>[2x]MLIIGERINGMFGDIKRAIQERDPAPVQEWARRQEEGGARALDLNVGPAVQDKVSAMEWLVEVTQEVSNLTLCLDSTNIKAIEAGLKKCKNRA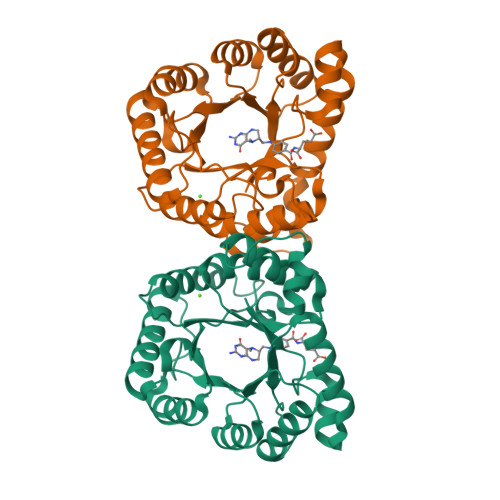MINSTNAEREKVEKLFPLAVEHGAALIGLTMNKTGIPKDSDTRLAFAMELVAAADEFGLPMEDLYIDPLILPANVAQDHAPEVLKTLQQIKMLADPAPKTVLGLSNVSQNCQNRPLINRTFLAMAMACGLDAAIADACDEALIETAATAEILLNQTVYCDSFVKMFKTR Sa-(+)-(6-(aminomethyl)-5-(2,4-dichlorophenyl)-7-methylimidazo[1,2-a]pyrimidin-2-yl)(morpholino)methanone | C19 H19 Cl2 N5 O2 | 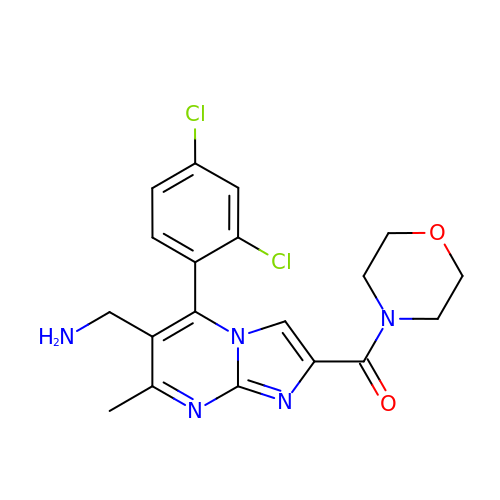MNRQGIJBOGTUFQ-UHFFFAOYSA-N>[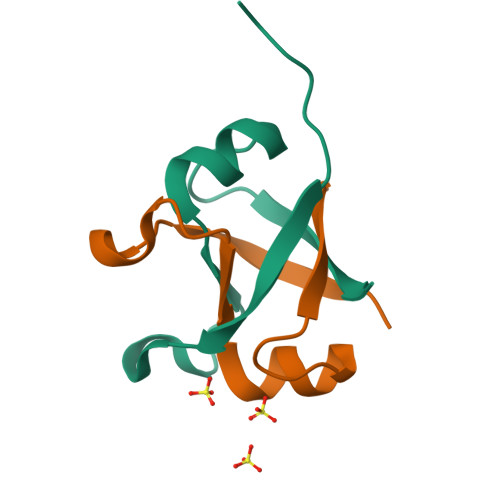4x]GPMPGKSVVARVAEAYPEDVGKRIVRMDKYERAKLGVSVGDYVEVKKV7-(4-{[3-(2,6-dimethylphenyl)-5-(1-methylethyl)isoxazol-4-yl]methoxy}phenyl)isoquinoline-3-carboxylic 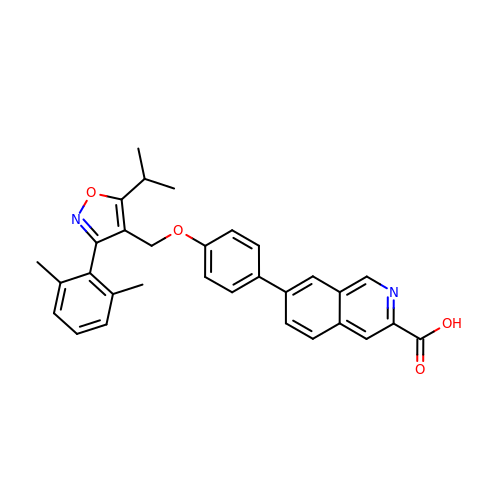acid | C31 H28 N2 O4 | DWPOYLMUSLXOEM-UHFFFAOYSA-N>MWKQNKDGIWYKAEHASFTVTAPEGIITRYKGPWTGHPQAGVLQKGQ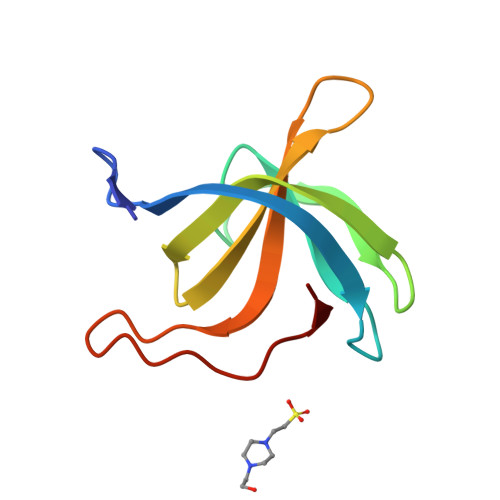TIKYDEVQKFDGHVWVSWETFEGETVYMPVRTWDAKTGKVGKLWGEIK[8x]>[2x]GPSASSTQKPAIVQEEEDLTASWTYFTKLDAQHTDDNNLFYSNIDEVLFYMNYRYDDFKLLDMDSTGTKNFETILSELWTALNGK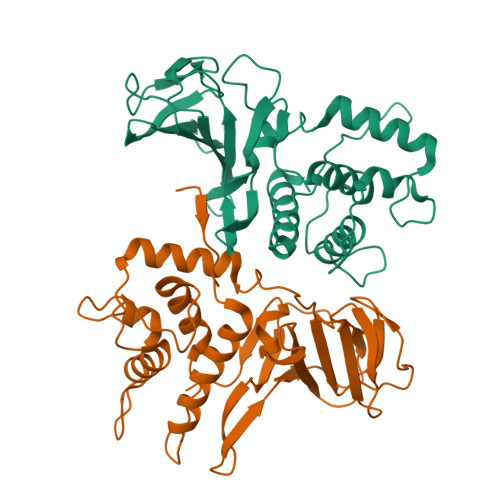KPDYQLKTMQSLETDKKSSYFIEEEQAKHYQEIKKELGYQTLDDLLSFPVKTDALIVNKRYGYDKSKEKLTLYQGIDVLIEDNQPFHSPMNGQIVSVPDTETLVIEKEKVARLTIRGVNTLRLTKGMDVEEGTFLGNTKNSTVTFQYEKYKKETKDWFFVNPAFYFPRVTYTQTTA>[2x]HHHHHHATLPAGASQVPTTPAGRPMPYAIRPMPEDRRFGYAIVGLGKYALNQILPGFAGCQHSRIEALVSGNAEKAKIVAAEYGVDPRKIYDYSN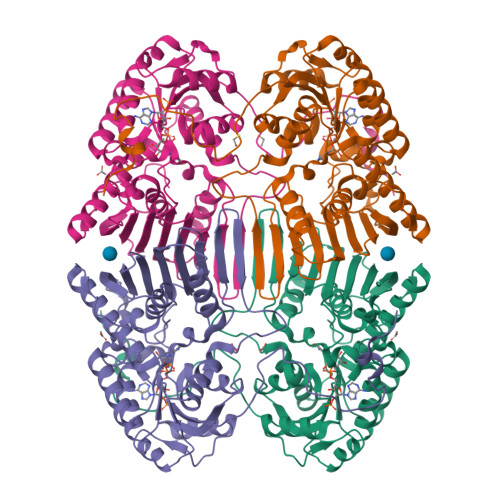FDKIAKDPKIDAVYIILPNSLHAEFAIRAFKAGKHVMCEKPMATSVADCQRMIDAAKAANKKLMIGYRCHYDPMNRAAVKLIRENQLGKLGMVTTDNSDVMDQNDPAQQWRLRRELAGGGSLMDIGIYGLNGTRYLLGEEPIEVRAYTYSDPNDERFVEVEDRIIWQMRFRSGALSHGASSYSTTTTSRFSVQGDKAVLLMDPATGYYQNLISVQTPGHANQSMMPQFIMPANNQFSAQLDHLAEAVINNKPVRSPGEEGMQDVRLIQAIYEAARTGRPVNTDWGYVRQGGY>METDLNSQDRKDLDKFIKFFALKTVQVIVQARLGEKICTRSSSSPTGSDWFNLAIKDIPEVTHEAKKALAGQLPAVGRSMCVEISLKTSEGDSMELEIWCLEMNEKCDKEIKVSYTVYNRLSLLLKSLLAITRVTPAYRLSRKQGHEYVILYRIYFGEVQLSGLGEGFQTVRVGTVGTPVGTITLSCAYR[2x];>[2x]MNCRSEVLEVSVEGRQVEEAMLAVLHTVLLHRSTGKFHYAAAGTYSIGTVGTQDVDCDFIDFTYVRVSSEELDRALRKVVGEFKDALRNSGGDGLGQMSLEFYQKKKSRWPFSDECIPWEVWTVKVHVVALATEQERQICREKVGEKLCEKIINIVEVMNRHEYLPKM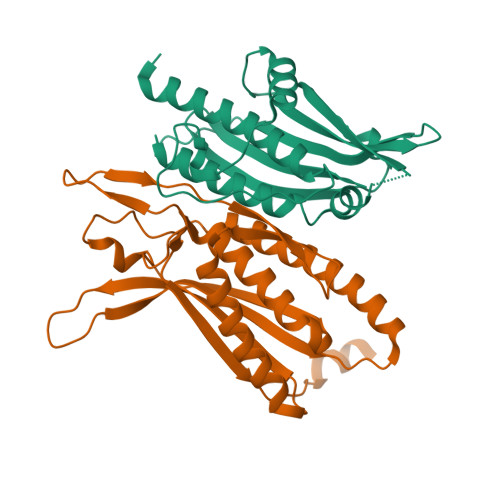PTQSEVDNVFDTGLRDVQPYLYKISFQITDALGTSVTTTMRRLIKDTLAL> GNDYICNKYKNIHDRMKKNNGNFVTDNFVKKSWEISNGVLIPPRRKNLFLYIDPSKICEYKKDPKLFKDFIYWSAFTEVERLKKA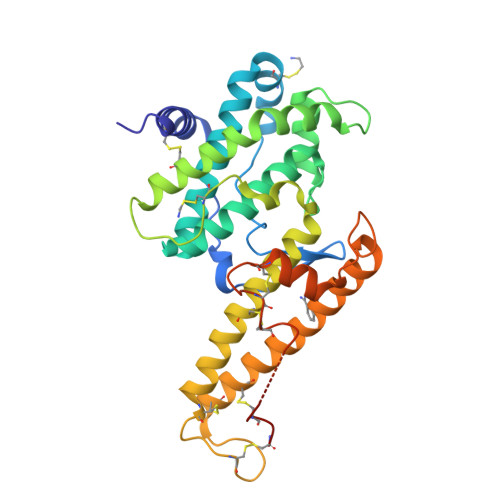YGGARAKVVHAMKYSFTDIGSIIKGDDMMEKNSSDKIGKILGDTDGQNEKRKKWWDMNKYHIWESMLCGYREAEGDTETNENCRFPDIESVPQFLRWFQEWSENFCDRRQKLYDKLNSECISAECTNGSVDNSKCTHACVNYKNYILTKKTEYEIQTNKYDNEFKNKNSNDKDAPDYLKEKCNDNKCECLNKHIDDKNKTWKNPYETLEDTFKSKCDCPKP> MPKALRFLGWPVLVGVLLALLIIQHNPELVGLPRQEVHVEQAPLLSRLQEGPPSYANAVSRAAPAVANLYTTKMVSKPSHPLFDDPMFRRFFGDNLPQQKRMESSLGSAVIMSAEGYLLTNNHVTAGADQIIVALRDGRETIAQLVGSDPETDLAVLKIDLKNLPAMTLGRSDGIRTGDVCLAIGNPFGVGQTVTMGIISATGRNQLGLNTYEDFIQTDAAINPGNSGGALVDAAGNLIGINTAIFSKSGGSQGIGFA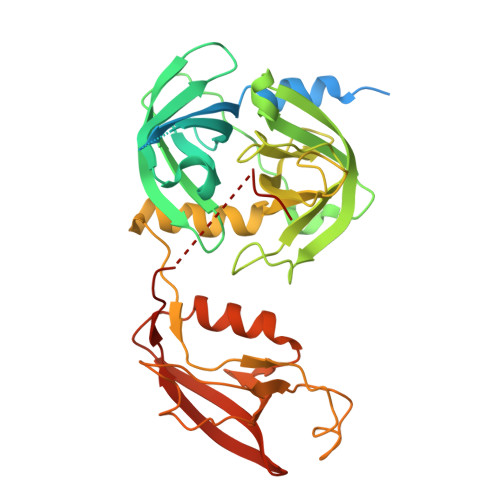IPTKLALEVMQSIIEHGQVIRGWLGVEVKALTPELAESLGLGETAGIVVAGVYRDGPAARGGLLPGDVILTIDKQEASDGRRSMNQVARTRPGQKISIVVLRNGQKVNLTAEVGLRPPPAPAPQQKQDGGE> DWVIPPINLPENSRGPFPQELVRIRSDRDKNLSLRYSVTGPGADQPPTGIFIINPISGQLSVTKPLDRELIARFHLRAHAVDINGNQVENPIDIVINVIDMNDNRPEFLHQVWNGSVPEGSKPGTYVMTVTAIDADDPNALNGML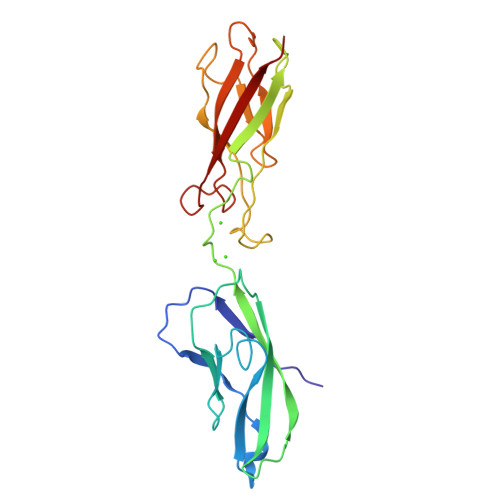RYRILSQAPSTPSPNMFTINNETGDIITVAAGLDREKVQQYTLIIQATDMEGNPTYGLSNTATAVITVTD>DAKAATKLADGKYNIAFTVWKGDKDESSRMNRYFESPATLTVKNGKQYVSFKVKDSTSIKSFQVEKDGQFVETTVLSENKKDNTRVVEFEVADLSKKLNGKVKINIPIINYNASYDIRFVF[2x]

B. anthracis, a Gram-positive pathogen that is a potential weapon for bioterrorism, secretes two hemophores (IsdX1 and IsdX2), that acquire heme from hemoglobin and promote bacterial growth in low-iron environments. The NEAT domain of IsdX1 is the only known NEAT domain to bind both heme and hemoglobin, as well as acquire heme from hemoglobin, thus making IsdX1 a useful model protein to study the relationship of these processes to one another. The structure consists of an immunoglobulin-like fold with eight β-strands arranged in two antiparallel β-sheets of a β-sandwich. The heme-binding pocket is enclosed primarily by a 310-helix (residues Arg-54 to Tyr-58) on one side of the heme and a long β-hairpin (β7–β8) on the other.

To gain an appreciation of the residues in IsdX1 necessary for the hemophore activity of this protein, we solved the crystal structure of apo-IsdX1 to 1.8 Å resolution. Overall, the backbone structure of IsdX1 is similar to the solved structures of NEAT domains from S. aureus, albeit with a unique surface charge distribution close to the heme binding pocket. The backbone of the 310-helix in IsdX1 is fairly well-ordered even in the absence of heme. The integrity of the 310-helix without heme could be due to the hydrogen bonding network between Ser-52, Ser-53, Arg-54 and Asn-56 and Met-55 from the helix making van der Waals contacts with residues in β4, β7, and β8. The structures of apo-IsdX1 and holo-IsdX1 are highly similar with RMSD of 0.51 Å. However, superimposition of both apo and holo structures highlight subtle residue sidechain conformational differences surrounding the heme binding site. Additionally, there is observable electron density for two side chain conformations for Met-55 within the apo structure, where one conformation is pointing toward the center of the heme binding pocket and the other away into the interior of IsdX1. In contrast, there is no conformational change observed for either Ser-52 or Ser-53 between the holo and apo structures. The apo-IsdX1 structure also has a similar protein interface near the vicinity of the heme-binding sites of adjacent monomers; however due to the lack of heme, there are more protein interactions between loop regions surrounding the active site.>MVAKEWQENKSWNAHFTEHKSQGVVVLWNENKQQGFTNNLKRANQAFLPASTFKIPNSLIALDLGVVKDEHQVFKWDGQTRDIATWNRDHNLITAMKYSVVPVYQEFARQIGEARMSKMLHAFDYGNEDISGNVDSFWLDGGI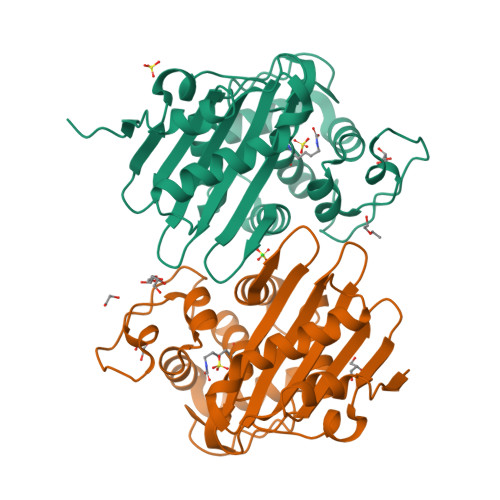RISATEQISFLRKLYHNKLHVSERSQRIVKQAMLTEANGDYIIRAKTGYSTKPKIGWWVGWVELDDNVWFFAMNMDMPTSDGLGLRQAITKEVLKQEKIIPFEHHHHHHHH[4x]> MSNKKQSNRLTEQHKLSQGVIGIFGDYAKAHDLAVGEVSKLVKKALSNEYPQLSFRYRDSIKKTEINEALKKIDPDLGGTLFVSNSSIKPDGGIVEVKDDYGEWRVVLVAEAKHQGKDIINIRNGLLVGKRGDQDLMTAGNAIERSHKNISEIANFMLSESHFPYVLFLEGSNFLTENISITRPDGRVVNLEYNSGILNRLDRLTAANYGMPI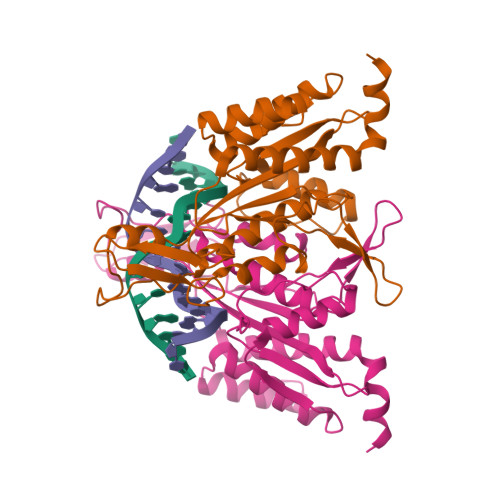NSNLCINKFVNHKDKSIMLQAASIYTQGDGREWDSKIMFEIMFDISTTSLRVLGRDLFEQLTSK> SPQPLEQIKLSESQLSGRVGMIEMDLASGRTLTAWRADERFPMVSTFKVVLCGAVLARVDAGDEQLERKIHYRQQDLVDYSPVSEKHLADGMTVGELCAAAITMSDNSAANLLLATVGGPAGLTAFLRQIGDNVTRLDRWATELNEALPGDARDTTTPASMAATLRKLLTSQRLSARSQRQLLQWMVDDRVAGPLIRSVLPAGWFIADKTGAGERGARGIVALLGPNNKAERIVVIYLRDTPASMAERNQQIAGIGAALIEH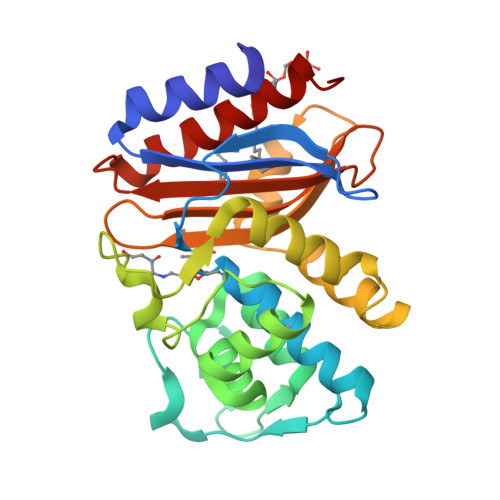WQR>[2x]MTATNKQVILKDYVSGFPTESDFDFTTTTVELRVPEGTNSVLVKNLYLSCDPYMRIRMGKPDPSTA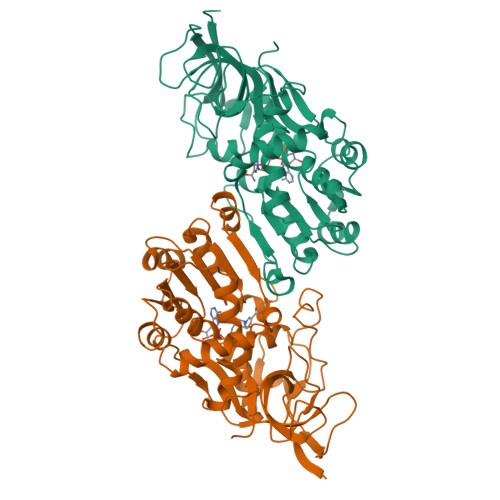ALAQAYTPGQPIQGYGVSRIIESGHPDYKKGDLLWGIVAWEEYSVITPMTHAHFKIQHTDVPLSYYTGLLGMPGMTAYAGFYEVCSPKEGETVYVSAASGAVGQLVGQLAKMMGCYVVGSAGSKEKVDLLKTKFGFDDAFNYKEESDLTAALKRCFPNGIDIYFENVGGKMLDAVLVNMNMHGRIAVCGMISQYNLENQEGVHNLSNIIYKRNRIQGFVVSDFYDKYSKFLEFVLPHIREGKITYVEDVADGLEKAPEALVGLFHGKNVGKQVVVVARE> SNARTITYDVFLSFRGEDTRFNFTDHLYSALGRRGIRTFR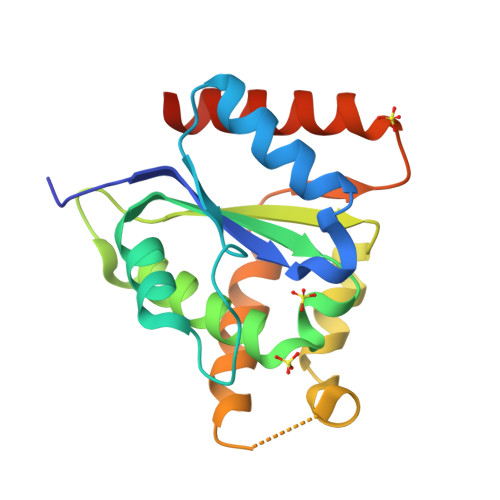DDKLRRGEAIAPELLKAIEESRSSVIVFSENYARSRWCLDELVKIMECHKDKKDPGHAVFPIFYHVDPSHVRKQEGSFGEAFAGYGENLKDKIPRWRTALTEAANLSGWPLQDGYESNQIKEITDSIFRRLKCKRLDAG> MSASRKTLVVTNDFPPRIGGIQSYLRDFIATQDPESIVVFASTQNAEEAHAYDKTLDYEVIRWPRSVMLPTPTTAHAMAEIIREREIDNVWFGAAAPLALMAGT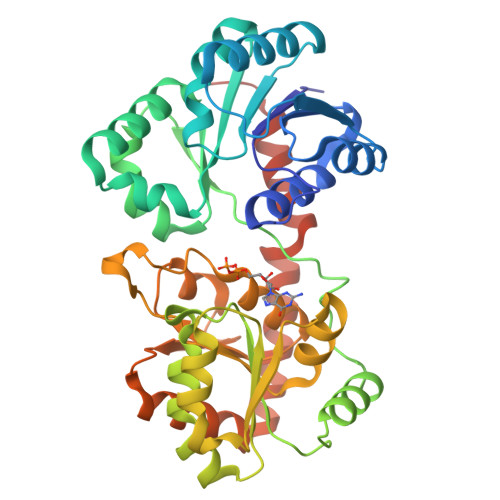AKQAGASKVIASTHGHEVGWSMLPGSRQSLRKIGTEVDVLTYISQYTLRRFKSAFGSHPTFEHLPSGVDVKRFTPATPEDKSATRKKLGFTDTTPVIACNSRLVPRKGQDSLIKAMPQVIAARPDAQLLIVGSGRYESTLRRLATDVSQNVKFLGRLEYQDMINTLAAADIFAMPARTRGGGLDVEGLGIVYLEAQACGVPVIAGTSGGAPETVTPATGLVVEGSDVDKLSELLIELLDDPIRRAAMGAAGRAHVEAEWSWEIMGERLTNILQSEPRKLAAALEHHHHHH>GGSHMELPGSSMKPSG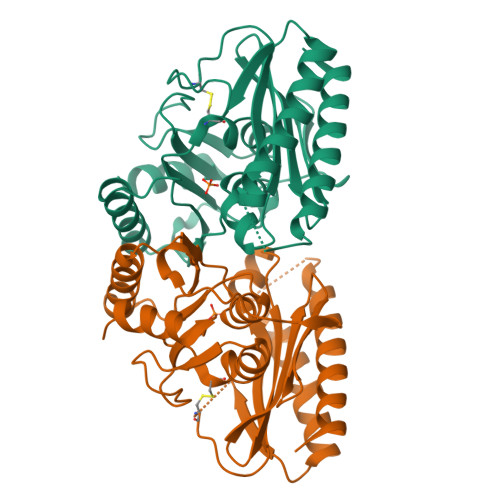EDQAALAAGPWEECFQAAVQLALRAGQIIRKALTEEKRVSTKTSAADLVTETDHLVEDLIISELRERFPSHRFIAEEAAASGAKCVLTHSPTWIIDPIDGTCNFVHRFPTVAVSIGFAVRQELEFGVIYHCTEERLYTGRRGRGAFCNGQRLRVSGETDLSKALVLTEIGPKRDPATLKLFLSNMERLLHAKAHGVRVIGSSTLALCHLASGAADAYYQFGLHCWDLAAATVIIREAGGIVIDTSGGPLDLMACRVVAASTREMAMLIAQALQTINYGRDDEK[2x]> MAIEQKLMDDHHEVDPRFPHHHPRPQSFWEARAKALE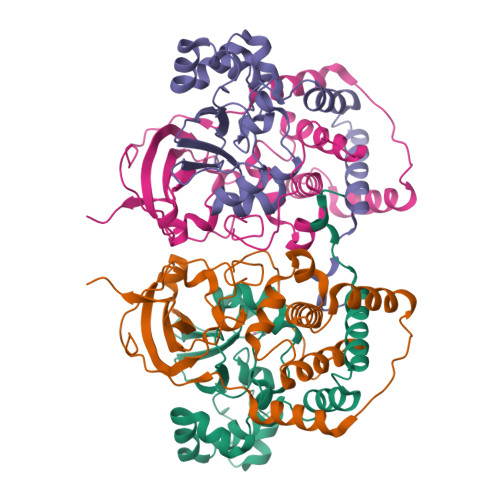SLLIEKRLLSSDAIERVIKHYEHELGPMNGAKVVAKAWTDPEFKQRLLEDPETVLRELGYFGLQGEHIRVVENTDTVHNVVVCTLCSCYPWPLLGLPPSWYKEPAYRSRVVKEPRKVLQEFGLDLPDSVEIRVWDSSSEVRFMVLPQRPEGTEGMTEEELAQIVTRDSMIGVAKVQPPKVIQE;> MNGIHDVGGMDGFGKIMYVKEEEDTYFKHDWERLTFGLVAGCMAQGLGMKAFDEFRIGIEKMRPVDYLTSSYYGHWIATVAYNLLETGVLDEKELEDRTQAFMEKPDTKIQRWENPKLVKVVEKALLEGLSPVREVSSFPRFEVGERIKTRNIHPTGHTRFPRYVRDKYGVIEEVYGAHVFPDDAAHRKGENPQYLYRVRFDAEELWGVKQNDSVYIDLWEGYLEPVSH methyl hydrogen (R)-hexylphosphonate | C7 H17 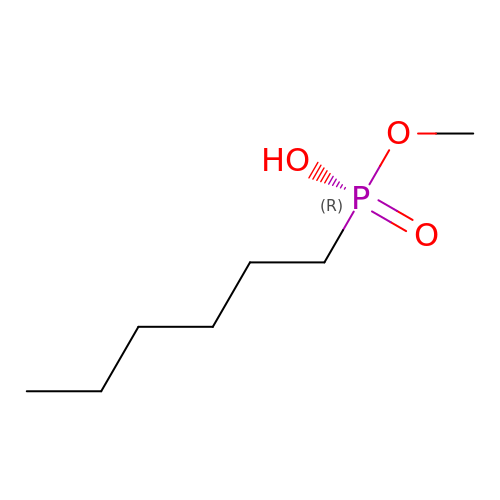O3 P | FOQQOPHBXMFLMD-UHFFFAOYSA-N> TGPAAQAAAAVQRVDGDFIRANAARTPDWPTIGVDYAETRYSRL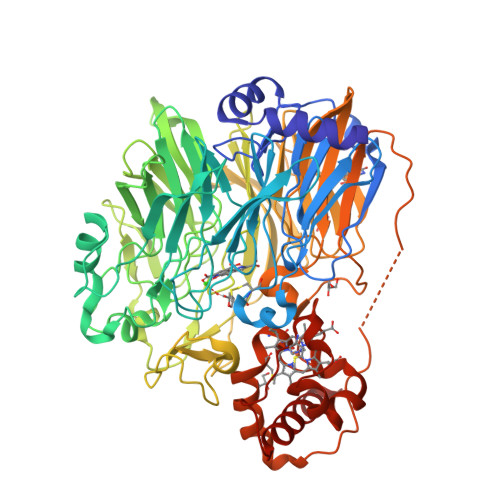DQINAANVKDLGLAWSYNLESTRGVEATPVVVDGIMYVSASWSVVHAIDTRTGNRIWTYDPQIDRSTGFKGCCDVVNRGVALWKGKVYVGAWDGRLIALDAATGKEVWHQNTFEGQKGSLTITGAPRVFKGKVIIGNGGAEYGVRGYITAYDAETGERKWRWFSVPGDPSKPFEDESMKRAARTWDPSGKWWEAGGGGTMWDSMTFDAELNTMYVGTGNGSPWSHKVRSPKGGDNLYLASIVALDPDTGKYKWHYQETPGDNWDYTSTQPMILADIKIAGKPRKVILHAPKNGFFFVLDRTNGKFISAKNFVPVNWASGYDKHGKPIGIAAARDGSKPQDAVPGPYGAHNWHPMSFNPQTGLVYLPAQNVPVNLMDDKKWEFNQAGPGKPQSGTGWNTAKFFNAEPPKSKPFGRLLAWDPVAQKAAWSVEHVSPWNGGTLTTAGNVVFQGTADGRLVAYHAATGEKLWEAPTGTGVVAAPSTYMVDGRQYVSVAVGWGGVYGLAARATERQGPGTVYTFVVGGKARMPEFVAQRTGQLLQGVKYDPAKVEAGTMLYVANCVFCHGVPGVDRGGNIPNLGYMDASYIENLPNFVFKGPAMVRGMPDFTGKLSGDDVESLKAFIQGTADAIRPKP> GMPALITYRTTVQEDWVDYNGHLRDAFYLLIFSYATDALMDRIGLDADSRGQSGNSLFTLEAHINYLHEVKLGTEVWVQT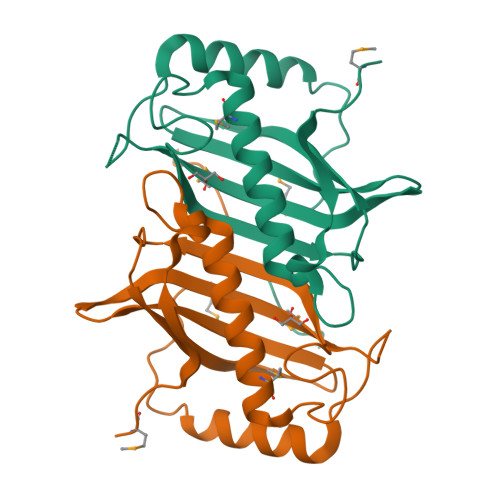QILGFDRKRLHVYHSLHRAGFDEVLAASEQMLLHVDLAGPQSAPFGHTTVCRLNHLVEQQEGAQAPQYMGRTIKLPA> HSSN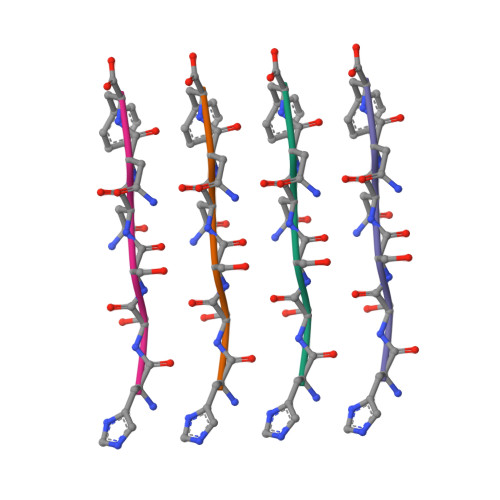NF> GGSEVRILLLGLDNAGKTTLLKQLASEDISHITPTQGFNIKSVQSQGFKLNVWDIGGQRKIRPYWRSYFENTDILIYVIDSADRKRFEETGQELTELLEEEKLSCVPVLIFANKQDLLTAAPASEIAEGLNLHTIRDRVWQIQSCSALTGEGVQDGMNWVCKNV;> GSMGCFFSKRRKADKESRPENEEERPKQYSWDQREKVDPKDYMFSGLKDETVGRLPGTVAGQQFLIQDCENCNIYIFDHSATVTIDDCTNCI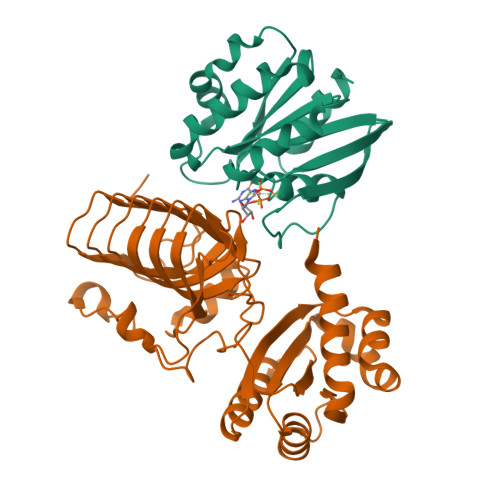IFLGPVKGSVFFRNCRDCKCTLACQQFRVRDCRKLEVFLCCATQPIIESSSNIKFGCFQWYYPELAFQFKDAGLSIFNNTWSNIHDFTPVSGELNWSLLPEDAVVQDYVPIPTTEELKAVRVSTEANRSIVPISRGQRQKSSDESCLVVLFAGDYTIANARKLIDEMVGKGFFLVQTKEVSMKAEDAQRVFREKAPDFLPLLNKGPVIALEFNGDGAVEVCQLIVNEIFNGTKMFVSESKETASGDVDSFYNFADIQMGI>[6x]HHLKPEMIEKLNEQMNLELYASLLYQQMSAWCSYHTFEGAAAFLRRHAQEEMTHMQRLFDYLTDTGNLPRINTVESPFAEYSSLDELFQETYKHEQLITQKINELAHAAMTNQDYP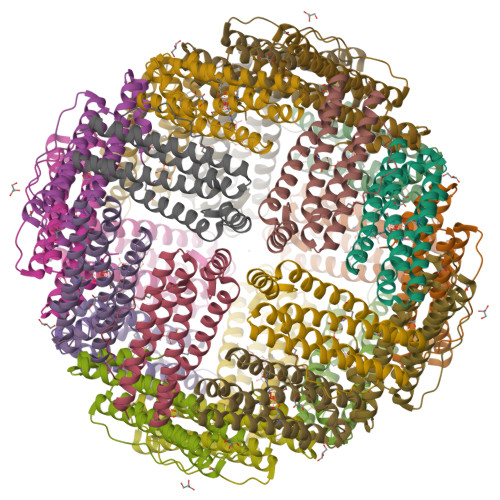TFNFLQWYVSEQHEEEKLFKSIIDKLSLAGKSGEGLYFIDKELSTLDTQN>MALQAASLVSSAFSVRKDAKLNASSSSFKDSSLFGASITDQIKSEHGSSSLRFKREQSLRNLAIR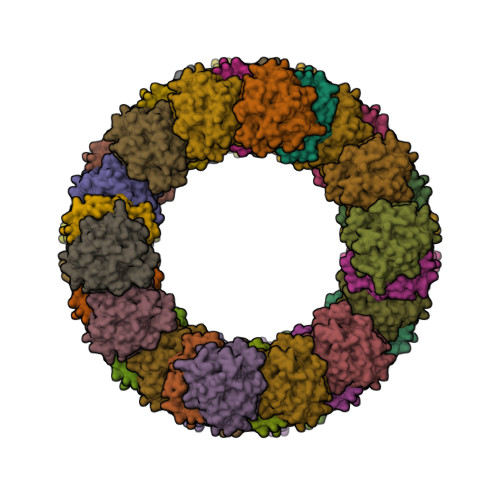AQTAATSSPTVTKSVDGKKTLRKGNVVVTGASSGLGLATAKALAETGKWNVIMACRDFLKAERAAKSVGMPKDSYTVMHLDLASLDSVRQFVDNFRRTETPLDVLVCNAAVYFPTAKEPTYSAEGFELSVATNHLGHFLLARLLLDDLKKSDYPSKRLIIVGSITGNTNTLAGNVPPKANLGDLRGLAGGLNGLNSSAMIDGGDFDGAKAYKDSKVCNMLTMQEFHRRFHEETGVTFASLYPGCIASTGLFREHIPLFRALFPPFQKYITKGYVSETESGKRLAQVVSDPSLTKSGVYWSWNNASASFENQLSEEASDVEKARKVWEISEKLVGLA[40x]>XEWEALEKKLAALESKCQALEKKLQALE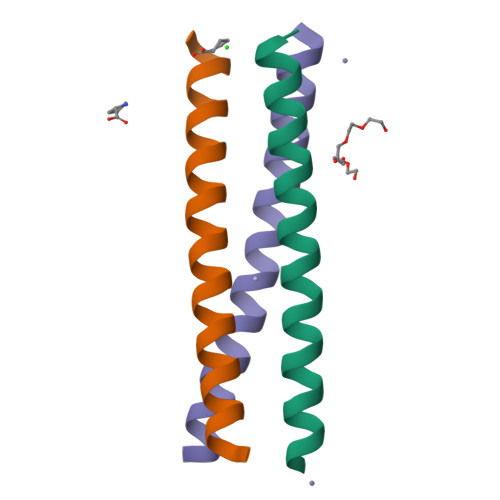KKLEALEHGX[3x]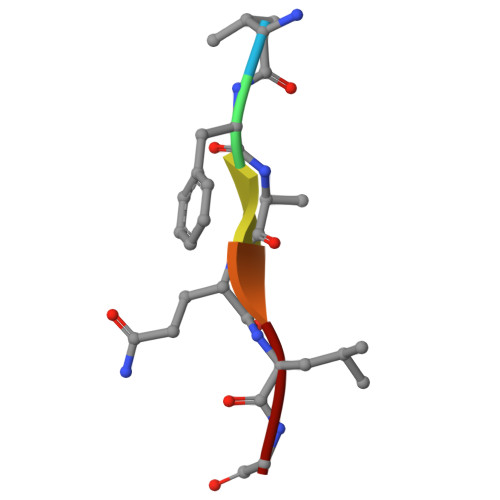> VFQQLG> MRFILVAVLAGLCAVSAISTSESSNYSQQQRDVWRLFKYINQPSYYKDHVEIAHSYYFYDHASNYAKHEVVEEFYRYFKYDTFLQRGEIFSVFHGEHLKQAIALFKLFYYANDFDTFYKTAVWARQHVNEGMFLYAFSVALIHRPDTYYFSLPPIYEIYPHYFYNYEVIQKAQHYKQMYYGQDGAHYNDRTIYANYSGYYVNVYPEQALAYFTEDVGVNSFYYYYNLYYPYWMSGEEFNLKYDNRGEIFYYMYQQILARYYLERLSHGFGEIDHFDWEVPFESGYYPSMCYPNGLYFPTRHAYAHLYEYFYNYGQHYGFNKYAHSYTHISDYERRIHDVIDSGYVHTHSGQKVDLFSHEGLDILGNLIEGNPESPYYHYYGAYQVFARHLLGYSHQPLTFHKLHPSALEHFETSMRDPAFYQLYKKLLGFFFRYKS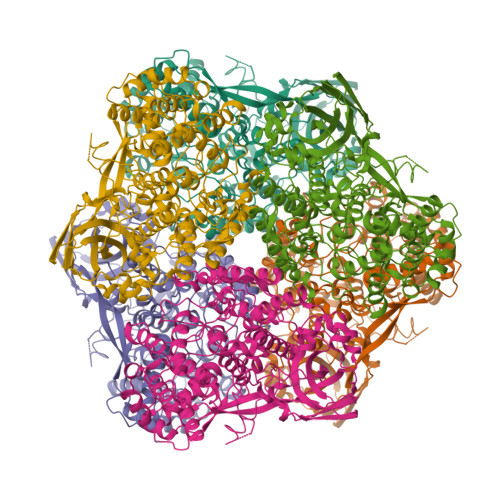QHYHYYDEHDLAYHGVHVKHVEVDPLVTYFDYFYADLSNAVYVTPEEFVHDSFKVHVAQERLNHKPFTYKIYIDSDKDTEAVVKVFLGPKYDEYGRYINLTENWMNFVQFDHFVYKLKSGENVISRNSHEIYNYIHDRTSYYELYQKAFGVYNKDQHFQFHDNQFFFGFPQRYMLPRGSPEGMTYQFYVFVTKYHPYKAHASVPMVGSGMHYVDAYPMGYPFDRPVYYEELFYALPNSYFQDVRIYYQGHNYEHHANHLIEM> IVGGYTCQENSVPYQVSLNSGYHFCGGSLINDQWVVSAAHCYKSRIQVRLGEHNINVLEGNEQFVNAAKIIKHPNFDRETYNNDIMLIK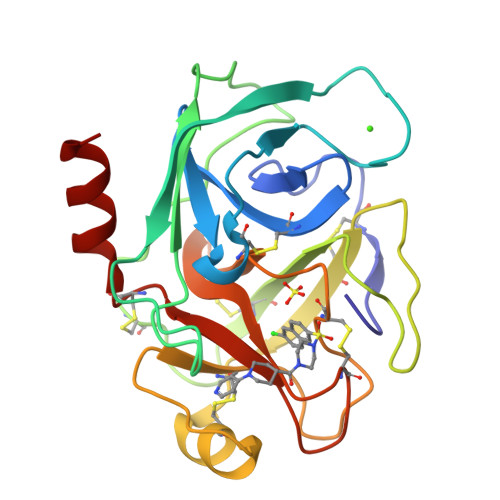LSSPVKLNARVATVALPSSCAPAGTQCLISGWGNTLSSGVNEPDLLQCLDAPLLPQADCEASSSFIITDNMVCVGFLEGGKDACQGDSGGPVVCNGELQGIVSWGYGCALPDNPGVYTKVCNYVDWIQDTIAAN>[2x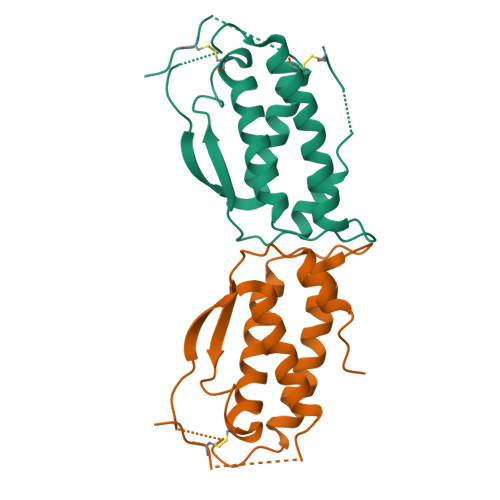]ICGNPVTDNVKDITKLVANLPNDYMITLNYVAGMDVLPSHCWLRDMVIQLSLSLTTLLDKFSNISEGLSNYSIIDKLGKIVDDLVLCMEENAPKNIKESPKRPETRSFTPEEFFSIFNRSIDAFKDFMVASDTSDCVLSHHHHHH> MAELRV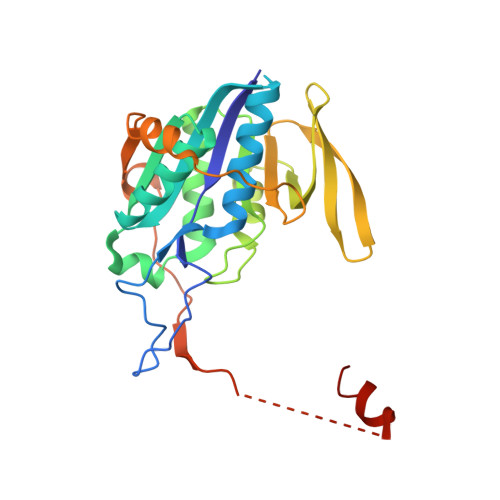LVAVKRVIDYAVKIRVKPDRTGVVTDGVKHSMNPFCEIAVEEAVRLKEKKLVKEVIAVSCGPAQCQETIRTALAMGADRGIHVEVPPAEAERLGPLQVARVLAKLAEKEKVDLVLLGKQAIDDDCNQTGQMTAGFLDWPQGTFASQVTLEGDKLKVERAIDGGLETLRLKLPAVVTADLRLNEPRYATLPNIMKAKKKKIEVIKPGDLGVDLTSKLSVISVEDPPQRTAGVKVETTEDLVAKLKEIGRI Among the five L,D-transpeptidase paralogs of M.tb, LdtMt2 plays an important role since an M.tb strain lacking the gene encoding this enzyme exhibits attenuation in virulence and exhibits enhanced susceptibility to β-lactam antibiotics. The L,D-transpeptidase class in M.tb is comprised of at least four substructural domains including two immunoglobulin-like domains (IgD1 and IgD2), a YkuD domain, and a C-terminal subdomain (CTSD). The YkuD domain has a highly conserved motif HXX14-17[S/T]HGChN containing three residues analogous to the catalytic triad of cysteine proteases: a cysteine, a histidine and a third residue (Cysteine 354, Histidine 336, and Serine 337 in LdtMt2) to catalyse the transpeptidation reaction. Based on our structural, biophysical, and biochemical data, we identify a new PG disaccharide moiety-binding pocket (named as S-pocket) at a distance of 21 Å from the catalytic site in LdtMt2.

To further understand the high-resolution details of structural changes may that occur in LdtMt2 upon covalent binding with β-lactam, the crystal structure of LdtMt2 was solved in complex with the experimental carbapenem drug T203 at a 1.7 Å resolution. Electron densities were observed in both the S-pocket and the outer cavity of catalytic pocket in the LdtMt2. Consistent with our docking results of T203 drug with LdtMt2, the 2-oxoethyl side-chain of R3 group from T203 could be modelled into the electron density of the S-pocket. A second T203 drug was also modelled into the electron density map of the catalytic pocket. In the S-pocket of LdtMt2, the 2-oxoethyl sidechain of T203 drug is stabilized through hydrophobic interactions with the A171, M157, P169, and L390 residues. No electron density was observed for the pyrrolidine ring of T203, while its carboxylic group fitted into an electron density making electrostatic interactions with backbone nitrogen of S296 and the guanidium side chain of R371. In the catalytic site, the T203 carbapenem interacts with the outer cavity at a covalent distance from the SΥ atom of C354. The amino N4 of the pyrrolidine ring makes electrostatic interactions with NE2 of H336 and the backbone amide nitrogen of H352. We observed that binding of the T203 drug introduces unique allosteric alterations in the salt bridge and hydrogen bond interactions spanning the entire distance from the S-pocket to the YkuD flap of the catalytic site. The T203 drug binding induces an additional alteration in the YkuD flap by breaking the hydrogen bond interactions of H300 with D323 as well as D321 and also the interactions between D304 and S306.

>GHMAPIKVIADKGTPFADLLVPKLTASVTDGAVGVTVDAPVSVTAADGVLAAVTMVNDNGRPVAGRLSPDGLRWSTTEQLGYNRRYTLNATALGLGGAATRQLTFQTSSPAHLTMPYVMPGDGEVVGVGEPVAIRFDENIADRGAAEKAIKITTNPPVEGAFYWLNNREVRWRPEHFWKPGTAVDVAVNTYGVDLGEGMFGEDNVQTHFTIGDEVIATADDNTKILTVRVNGEVVKSMPTSMGKDSTPTANGIYIVGSRYKHIIMDSSTYGVPVNSPNGYRTDVDWATQISYSGVFVHSAPWSVGAQGHTNTSHGCLNVSPSNAQWFYDHVKRGDIVEVVNTVGGTLPGIDGLGDWNIPWDQWRAGNAKA[2x]>GAKLNRKLRQDSTDRYKTKLYLWRNLGGLIPEDMAISVTESITADWKQYNDMMSKVRNETLDILKTNKVATEDYIGYIAFAEELAHQVWKNKNSSPDPNTANEASKTDLESK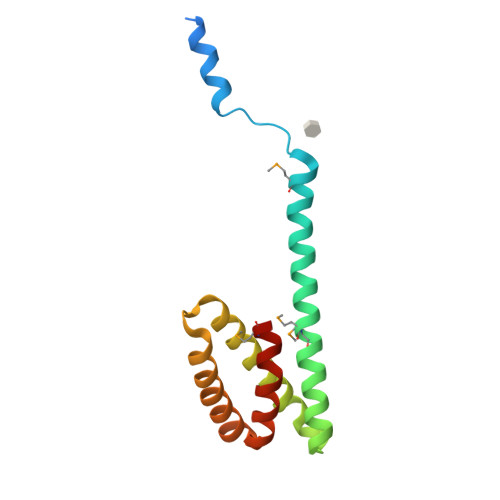YSDVYGLDVTVLDAIYNAVIPIIMGGGS[4x]>[8x]MKDGMRVGERFTHDFVVPPHKTVRHLYPESPEFAEFPEVFATGFMVGLMEWACVRAMAPYLEPGEGSLGTAICVTHTAATPPGLTVTVTAELR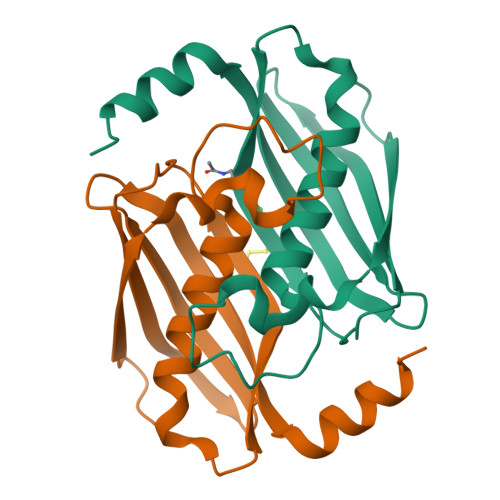SVEGRRLSWRVSAHDGVDEIGSGTHERAVIHLEKFNAKVRQKTPAG>MDSTGRAYDGASEFKSVLVTEGTSHYTPVEVYNILDELKTIKITSTIAEQSVVSRTPIPLSKIGLQDVKKLFDINVIKCGSSLRIVDEPQVTFIVSYAKDIYDKFMCIEHDSAYEPSLTMHRVRVIYSMLNDYCAKMISEVPYESSFVGELPVKSVTLNKLGDRNMDALAEHLLFEHDVVNAQRENRIFYQRKSAPAVPVIFGDDLEPAVRERANLYHRYSVPYHQIELALHALANDLLSIQYCHPTVVYNYLSSRAPNFLRLDDQVSLKLTSAGIGTLMPRPVVQLLDYDLVYMSPLALNNLASRLLRKISLHLVMQMVTAVQQDLGEVVSVSSNVTNPASACLVRMNVQGVQTLAVFIAQSMLNPNISYGMISGLTLDCFSNFIYGACLMLFQALIPPSALTARQRLDINNRFAYFLIKCHATQATTARLVANQVIYPVDAIDQWQSNGRDVLVAIYNNLLPGELVLTNLIQTYFRGNTAQQAAEILIPADQTSYGANETRALSAPYLFGAPINMLAPDARLSTYKRDLALPDRSPILITTVEGQNSISIENLRHKTGLIRAMYLNGFVTQPPAWIRNANSNTALLSRFLDATPNLLGIYEAILANTYANAVNVYCDSVYRADIPIEWKLHQSVDPQDLLFGVFGIVPQYQILNEAVPDFFAGGEDILILQLIRAVYDTLSNKLGRNPADIFHLEEVFKVIEEIVSVLVQQKIDVRKYFTESMRSGSFSKPRWDNFLRRPVAQRLPNLYSVIMTQADHVYNYMTQLTHIIPITDCFYIVKNSGFVDRGSTGPVIASSSVYENVLKVVHTIADFDAANALRLQRRRVDNTSYTDSLSDMFNGLRSISSSEFVRSVNGRSVFTEGRIDAIKVNMRAKFDLQFITEEGGYSKPPNVKKLMFSDFLSFLDSHKSDYRPPLLTVPITIGLNNLGETNSNTLRMRSEAIDEYFSSYVGAQILVPINVVDTRVYTEFSELRNFFTGDVVIRDDPFDVWDGVKATYIPIGVHGVRLDPNGDQPPL[2x];>MSRQMWLDTSALLEAISEYVVRCNGDTFSGLTTGDFNALSNMFTQLSVSSAGYVSDPRVPLQTMSNMFVSFITSTDRCGYMLRKTWFNSDTKPTVSDDFITTYIRPRLQVPMSDTVRQLNNLSLQPSAKPKLYERQNAIMKGLDIPYSEPIEPCKLFRSVAGQTGNIPMMGILATPPAAQQQPFFVAERRRILFGIRSNAAIPAGAYQFVVPAWASVLSVTGAYVYFTNSFFGTIIAGVTATATAADAATTFTVPTDANNLPVQTDSRLSFSLGGGNINLELGVAKTGFCVAIEGEFTILANRSQAYYTLNSITQTPTSIDDFDVSDFLTTFLSQLRACGQYEIFSDAMDQLTNSLITNYMDPPAIPAGLAFTSPWFRFSERARTILALQNVDLNIRKLIVRHLWVITSLIAVFGRYYRPN[13x];> MSAIVGLCLLSEKVVLSRSLTDEVSKLYKLNRGNVKEPRKYATERMSTQSKPVALQVPVSTIILDYKNEDFIKQNPTYSAMDIIGSPSNTAPQTAFQSIMPSLSALFNTPFIQGAFRHRIISSMGPEISYLVMVIGPPSGFMDTPNVSSAQSSVHTVSNADVDLNDIIAINSTMAKSTKLVSASTLQAMLVNDVYDRCMDLDGILLSQALPFFRNYVNVQSKGSLPPAVAACLNTPIKELFSMGSGKREPLALEFRKDNEGQCIGIVLPKGHEGDTLSSRYPAVFINESEPFSDKERSELSELKRTDSDAYEKLYSETISKHVSDGSYGNRVIISHKMSRLSNGGVKIIGRFKISDFNTVKKNLSSRSGEIDSAKEQWEALSGNGLVTDSNISMLHDKILDTITSNKPGVVLRDGNKKSENIVVCFKNGFPNKKHSLLQLTKNGISVVSLDELTDAGILVESTGPDRVRRSPKVLANKLSSFKGRKVTLDVDNMST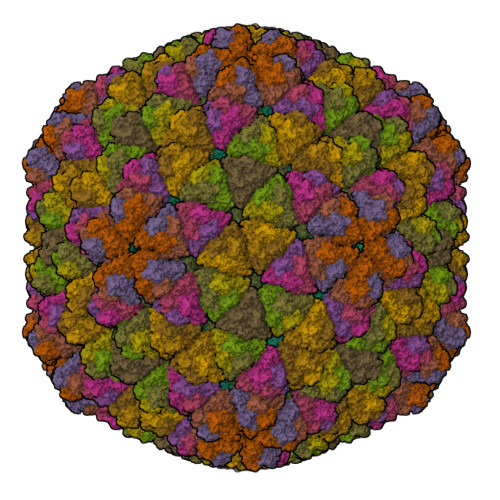EALIQKLSTL>[2x]MLRFVTKNSQDKSSDLFSICSDRGTFVAHNRVRTDFKFDNLVFNRVYGVSQKFTLVGNPTVCFNEGSSYLEGIAKKYLTLDGGLA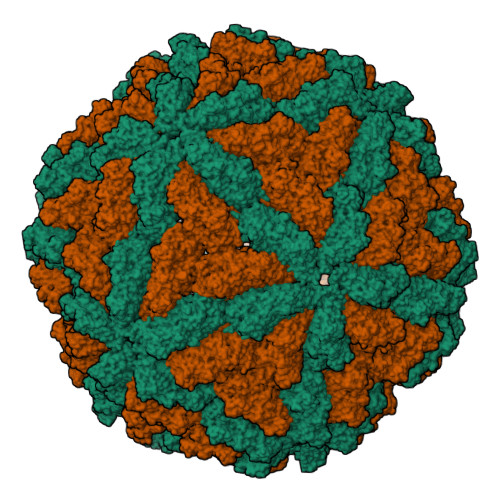IDNVLNELRSTCGIPGNAVASHAYNITSWRWYDNHVALLMNMLRAYHLQVLTEQGQYSAGDIPMYHDGHVKIKLPVTIDDTAGPTQFAWPSDRSTDSYPDWAQFSESFPSIDVPYLDVRPLTVTEVNFVLMMMSKWHRRTNLAIDYEAPQLADKFAYRHALTVQDADEWIEGDRTDDQFRPPSSKVMLSALRKYVNHNRLYNQFYTAAQLLAQIMMKPVPNCAEGYAWLMHDALVNIPKFGSIRGRYPFLLSGDAALIQATALEDWSAIMAKPELVFTYAMQVSVALNTGLYLRRVKKTGFGTTIDDSYEDGAFLQPETFVQAALACCTGQDAPLNGMSDVYVTYPDLLEFDAVTQVPITVIEPAGYNIVDDHLVVVGVPVACSPYMIFPVAAFDTANPYCGNFVIKAANKYLRKGAVYDKLEAWKLAWALRVAGYDTHFKVYGDTHGLTKFYADNGDTWTHIPEFVTDGDVMEVFVTAIERRARHFVELPRLNSPAFFRSVEVSTTIYDTHVQAGAHAVYHASRINLDYVKPVSTGIQVINAGELKNYWGSVRRTQQGLGVVGLTMPAVMPTGEPTAGAAHEELIEQADNVLVE> NLRGGAFVSNTQITMADKQKKFINEIQEGDLVRSYSITD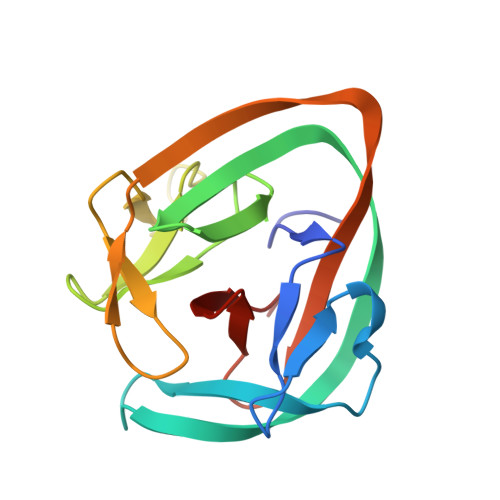ETFQQNAVTSIVKHEADQLCQINFGKQHVVCTVNHRFYDPESKLWKSVCPHPGSGISFLKKYDYLLSEEGEKLQITEIKTFTTKQPVFIYHIQVENNHNFFANGVLAHAMQ>[2x]SKI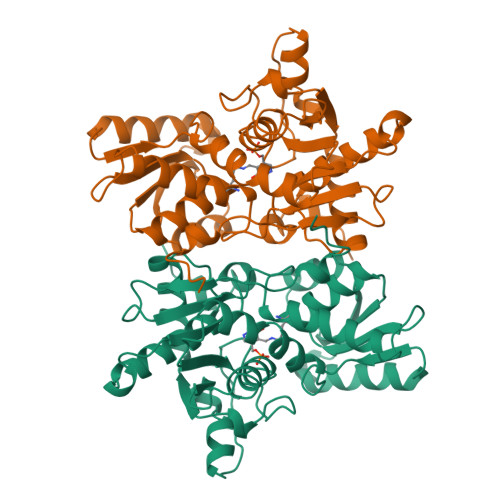YEDNSLTIGHTPLVRLNRIGNGRILAKVESRNPSFSVKCRIGANMIWDAEKRGVLKPGVELVEPTNGNTGIALAYVAAARGYKLTLTMPETMSIERRKLLKALGANLVLTEGAKGMKGAIQKAEEIVASDPQKYLLLQQFSNPANPEIHEKTTGPEIWEDTDGQVDVFISGVGTGGTLTGVTRYIKGTKGKTDLITVAVEPTDSPVIAQALAGEEIKPGPHKIQGIGAGFIPGNLDLKLIDKVVGITNEEAISTARRLMEEEGILAGISSGAAVAAALKLQEDESFTNKNIVVILPSSGERYLSTALFADLFTEKELQQ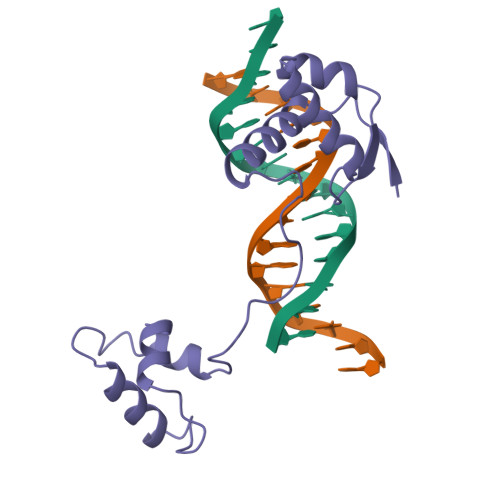> GQGRVNQLGGVFINGRPLPNNIRLKIVEMAADGIRPCVISRQLRVSHGCVSKILNRYQETGSIRPGVIGGSKPRIATPEIENRIEEYKRSSPGMFSWEIREKLIREGVCDRSTAPSVSAISRLVRGRD> SAQTIEATTVSQLEKAHVRIGDTLRLTGTGMCNIRTPGSWSAKEDSPFLPFDCSQIVWNDAPPLPLPESDIVSKATALMQSVQRQLHPETDDDSRVSPALRSAIQKSGMVLLDDFGDIVQKTNDLCSAKDDCLRLKNALVNLGNTRNWETLTKRATAGKLDGVNVLLRPVSAESLENLVTTSTAPFVIRETSRAAQALNSPAPGGFLIASDEGSVLVNQPWPAVSLYD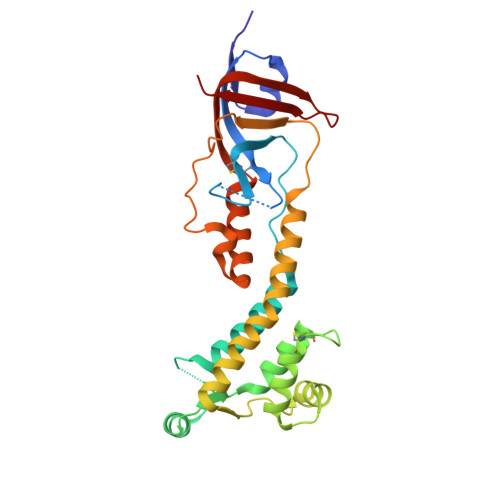YPAHEQWGELRRLAGMLMHTPFHAEGIVTNLFTDANGTQHINLHRI> QQCNGIYIWKIGNFGMHLKCQEEEKPVVIHSPGFYTGKPGYKLCMRLHLQLPTAQRCANYISLFVHTMQGEYDSHLPWPFQGTIRLTILDQSEAPVRQNHEEIMDAKPELLAFQRPTIPRNPKGFGYVTFMHLEALRQRTFIKDDTLLVRCEVSTR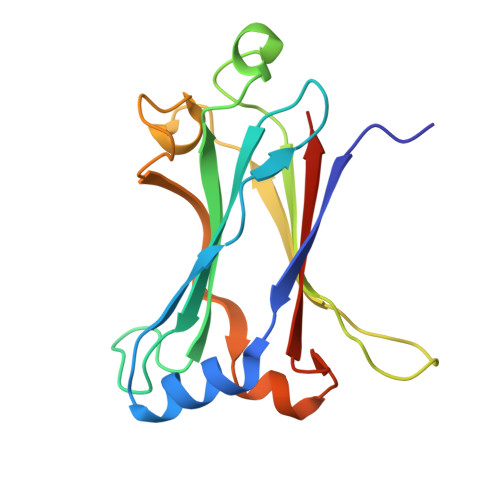FDLE> MEQAFLQDLDDFQAWLSITQKAVASEDMPESLPEAEQLLQQHAGIKDEIDGHQDSYQRVKESGEKVIQGQTDPEYLLLGQRLEGLDTGWDALGRMWESRSHTLAQCLGFQEFQKDAKQAEAILSNQEYTLAHLEPPDSLEAAEAGIRKFEDFLGSMENNRDKVLSPVDS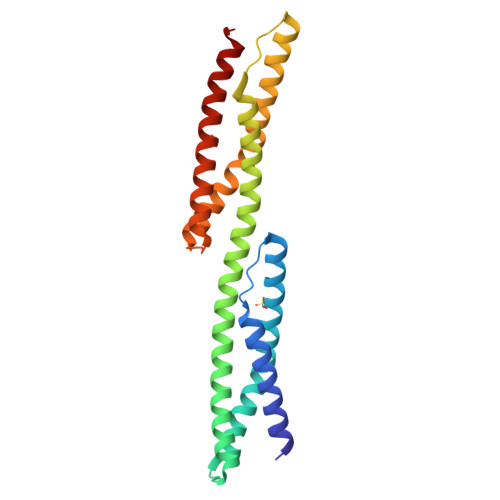GNKLVAEGNLYSDKIKEKVQLIEDRHRKNNEKAQEASVLLRDNLE>[6x]GLKEHDFNPEEAEETKQVSWKLVTEYAMETKCDDVLLLLGMYLEFQYSFEMCLKCIKKEQPSHYKYHEKHYANAAIFADSKNQKTICQQAVDTVLAKKRVDSLQLTREQMLTNRFNDLLDRMDIMFGSTGSADIEEWMAGVAWLHCLLPKMDSVVYDFLKCMVYNIPKKRYWLFKGP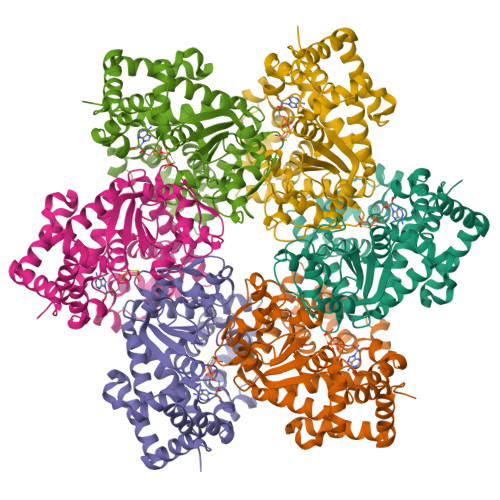IDSGKTTLAAALLELCGGKALNVNLPLDRLNFELGVAIDQFLVVFEDVKGTGGESRDLPSGQGINNLDNLRDYLDGSVKVNLEKKHLNKRTQIFPPGIVTMNEYSVPKTLQARFVKQIDFRPKDYLKHCLERSEFLLEKRIIQSGIALLLMLIWYRPVAEFAQSIQSRIVEWKERLDKEFSLSVYQKMKFNVAMGIGVLD>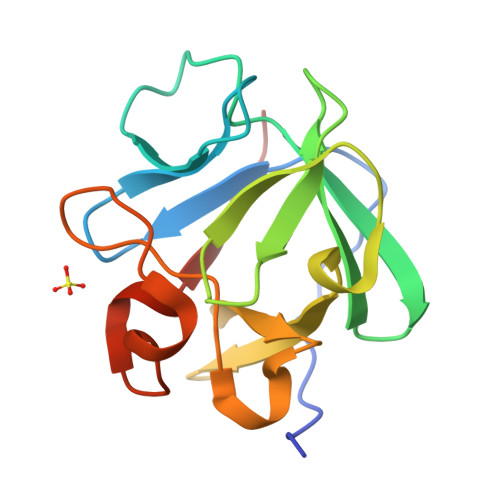HHHHHHFNLPPGNYKKPTLLYCSNGGHFLRILPDGTVDGTRDRSDQHIQLQLSAESVGEVYIKSTETGQYLAMDTDGLLYGSQTPNEECLFLERLEENHYNTYISKKHAEKNWFVGLKKNGSVKRGPRTHYGQKAILFLPLPVSSD[2x]> AGHMHPRPLPAAGLPGDLFGLGIASRIRTDSNSTAKAATDFGQMVRAAPEAVFHPATPADIAALVRFSATSAAPFPVAPRGQGHSWRGQALAPGGVVVDMGSLGRGPRINVSAATGAEPFVDAGGEQLWVDVLRATLRHGLAPRVWTDYLRLTVGGTLSNAGIGGQAFRHGPQIANVHELDVVTGTGEMVTCSMDVNSDLFMAALGGLGQFGVITRARIRLEP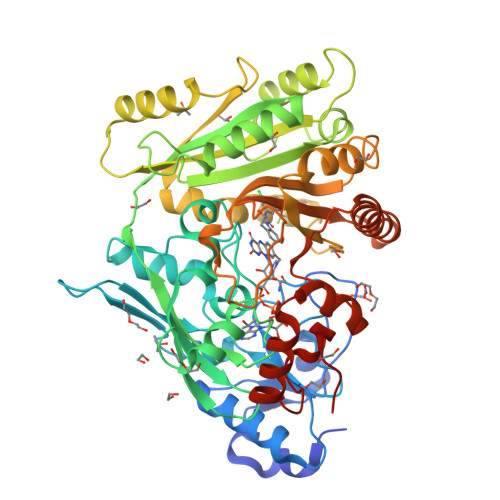APKRVRWVRLAYTDVATFTKDQEFLISNRTSQVGFDYVEGQVQLNRSLVEGPKSTPFFSGADLARLAGLASRTGPTAIYYIEGAMYYTEDTAISVDKKMKALLDQLSFEPGFPFTKDVTFVQFLDRVREEERVLRSAGAWEVPHPWLNLFVPRSRILDFDDGVFKALLKDANPAGIILMYPMNKDRWDDRMTAMTPATDDDDNVFYAVSFLWSALSADDVPQLERWNKAVLDFCDRSGIECKQYLPHYTSQDGWRRHFGAKWSRIAELKARYDPRALLSPGQRIFPVPVESSGIASA>[2x]MANPYERGPDPTESSIEAVRGPFAVAQTTVSRLQADGFGGGTIYYPTDTSQGTFGAVAISPGFTAGQESIAWLGPRIASQGFVVITIDTITRLDQPDSRGRQLQAALDHLRTNSVVRNRIDPNRMAVMG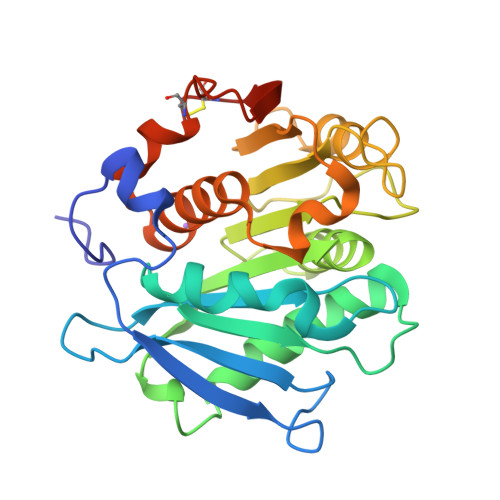HSMGGGGALSAAANNTSLEAAIPLQGWHTRKNWSSVRTPTLVVGAQLDTIAPVSSHSEAFYNSLPSDLDKAYMELRGASHLVSNTPDTTTAKYSIAWLKRFVDDDLRYEQFLCPAPDDFAISEYRSTCPFLEHHHHHH>ADPCPAPCSCAGTLVDCGRRGLTALPALPARTTELVLTGNNLTSVPPGAFDHLPQLRTAHLGANPWR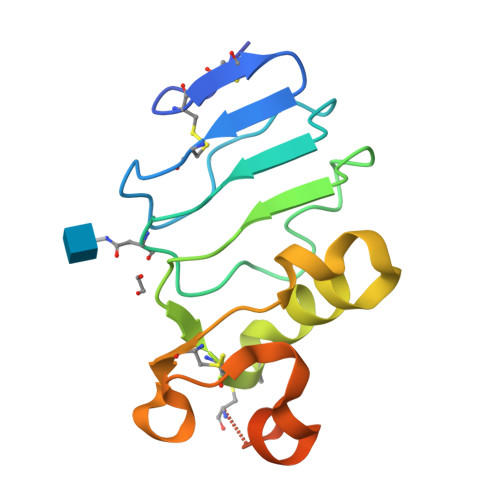CDCSLTYLRLWLEDRPERAPYRDLRCVAPPALRGRLLPYLAEDELRAACAPGPLSSHHHHHH[4x]(1R)-3-(2,4-diamino-6-methylpyrimidin-5-yl)-1-(3,4,5-trimethoxyphenyl)prop-2-yn-1-ol 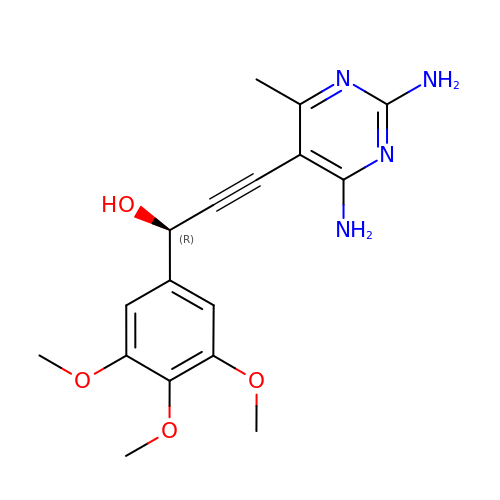| C17 H20 N4 O4 | MRGVCWULZNEIIL-LBPRGKRZSA-N> MSVNGNLRSLIDMLEAAQDGHMIKIALRSFAHSCGYDRFAYLQKDGTQVRTFHSYPGPWESIYLGSDYFNIDPVLAEAKRRRDVFFWTADAWPARGSSPLRRFRDEAIS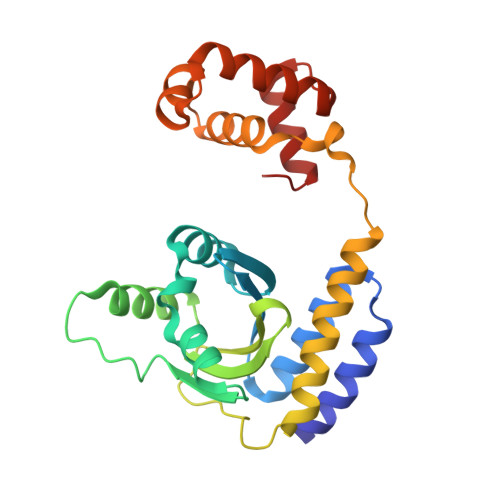HGIRCGVTIPVEGSYGSAMMLTFASPERKVDISGVLDPKKAVQLLMMVHYQLKIIAAKTVLNPKQMLSPREMLCLVWASKGKTASVTANLTGINARTVQHYLDKARAKLDAESVPQLVAIAKDRGLV>[6x]MFEIKKICCIGAGYVGGPTCSVIAHMCPEIRVTVVDVNESRINAWNSPTLPIYEPGLKEVVESCRGKNLFFSTNIDDAIKEADLVFISVNTPTKTYGMGKGRAADLKYIEACARRIVQNSNGYKIVTEKSTVPVRAAESIRRIFDANTKPNLNLQVLSNPEFLAEGTAIKDLKNPDRVLIGGDETPEGQRAVQALCAVYEHWVPREKILTTNTWSSELSKLAANAFLAQRISSINSISALCEATGADVEEVATAIGMDQRIGNKFLKASVGFGGSCFQKDVLNLVYLCEALNLPEVARYWQQVIDMNDYQRRRFASRIIDSLFNTVTDKKIAILGFAFKKDTGDTRESSSIYISKYLMDEGAHLHIYDPKVPREQIVVDLSHPGVSEDDQVSRLVTISKDPYEACDGAHAVVICTEWDMFKELDYERIHKKMLKPAFIFDGRRVLDGLHNELQTIGFQIETIGKKVSSKRIPYAPSGEIPKFSLQDPPNKKPKV

Human UDP-glucose dehydrogenase (hUGDH) catalyzes the oxidation of UDP-glucose into UDP-glucuronic acid, an essential substrate in the Phase II metabolism of drugs. hUGDH is a hexamer that exists in an equilibrium between an active (E) state and an inactive (EΩ) state, with the latter being stabilized by the binding of the allosteric inhibitor UDP-xylose (UDP-Xyl). hUGDH forms a hexamer arranged as a trimer of dimers, with each chain containing a NAD+ binding domain (NB domain) and a substrate binding domain (SB domain). The active site is located between the NB and SB domains within each chain, which are both flexible and undergo a rigid-body rotation to open the active site and bind substrate. What makes this allosteric is that the binding of UDP-Xyl changes the structure of the hexamer-building interface and increases the affinity between the adjacent subunits to form EΩ.12. This remarkable conformational change is controlled by a buried allosteric switch (the Thr131 loop/α6 helix) that responds to the identity of the C5 position of the nucleotide sugar bound in the active site.

Unliganded hUGDH (hUGDH) was purified and used to prepare electron microscopy grids for single particle cryo-EM data collection. Processing, refinement, and image reconstruction produced a 2.06 Å density map which revealed that the major class of unliganded hUGDH is the 32 symmetry E state. Analysis of the particle set with 2D classification shows that the E state represents ∼60% of the particles, with the remaining fraction appearing to represent dimers or monomers, which is consistent with sedimentation velocity data showing that the E state forms a less stable hexamer than the EΩ state. As expected, there is no evidence of a nucleotide sugar in the active sites (not shown). The cryo-EM structure also shows that all the NB domains are rotated 11.8° to the open conformation. The cryo-EM density of the open NB domains is less ordered than the rest of the structure, indicating domain flexibility. This is consistent with the various crystal structures of the E state, which reveal NB domain rotations ranging from 0 to 13°, depending on the unique packing constraints of the different crystal lattices. Additional evidence that unliganded hUGDH favors the E state can be observed in progress curve analysis, which shows that the unliganded enzyme no longer displays the hysteresis observed in hUGDH:UX4O. Since hysteresis is a result of the slow transition from the EΩ to the E state,14−16 the lack of a lag in unliganded hUGDH indicates the absence of a significant EΩ population and is consistent with the cryo-EM data we have presented thus far. Here, we show that UX4O shifts the ensemble toward the EΩ state, and that unliganded hUGDH strongly favors the E state.>MAASTPVVVDIHTHMYPPSYIAMLEKRQTIPLVRTFPQADEPRLILLSSELAALDAALADPAAKLPGRPLSTHFASLAQKMHFMDTNGIRVSVISLANPWFDFLAPDEAPGIADAVNAEFSDMCAQHVGRLFFFAALPLSAPVDAVKASIERVKNLKYCRGIILGTSGLGKGLDDPHLLPVFEAVADAKLLVFLAPHYGLPNEVYGPRSEEYGHVLPLALGFPMETTIAVARMYMAGVFDHVRNLQMLLAHSGGTLPFLAGRIESCIVHDGHLVKTGKVPKDRRTIWTVLKEQIYLDAVIYSEVGLQAAIASSGADRLMFGTDHPFFPPIEEDVQGP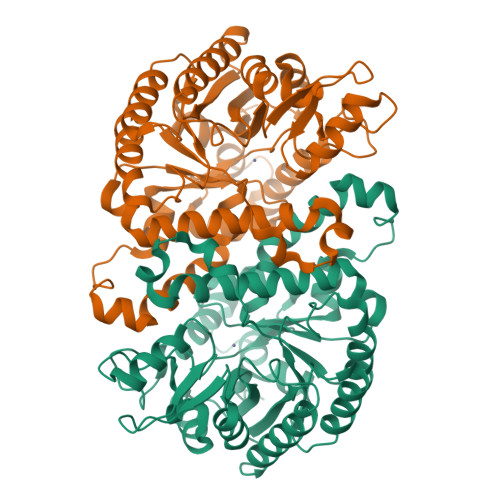WDSSRLNAQAVIKAVGEGSSDAAAVMGLNAVRVLSLKAE[2x]> WMLKLIVKNGYVIDPSQNLEGEFDILVENGKIKKIDKNILVPEAEIIDAKGLIVCPGFIDIHVHLRDPGQTYKEDIESGSRCAVAGGFTTIVCMPNTNPPIDNTTVVNYILQKSKSVGLCRVLPTGTITKGRKGKEIADFYSLKEAGCVAFTDDGSPVMDSSVMRKALELASQLGVPIMDHCEDDKLAYGVINEGEVSALLGLSSRAPEAEEIQIARDGILAQRTGGHVHIQHVSTKLSLEIIE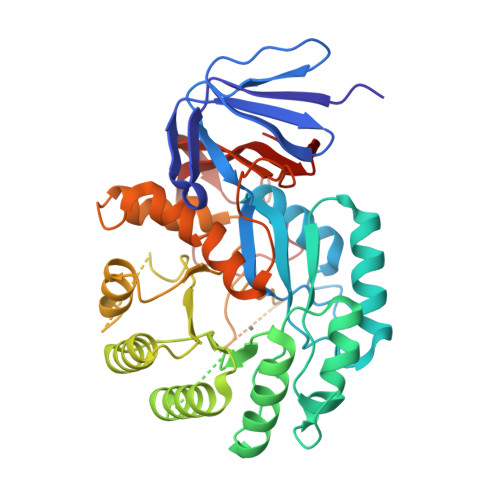FFKEKGVKITCEVNPNHLLFTEREVLNSGANARVNPPLRKKEDRLALIEGVKRGIIDCFATDHAPHQTFEKELVEFAMPGIIGLQTALPSALELYRKGIISLKKLIEMFTINPARIIGVDLGTLKLGSPADITIFDPNKEWILNEETNLSKSRNTPLWGKVLKGKVIYTIKDGKMVYKD>[4x]MKLVATLSSPEELELAEKADVVELRIDLFDFSGARVDKEKILTCRR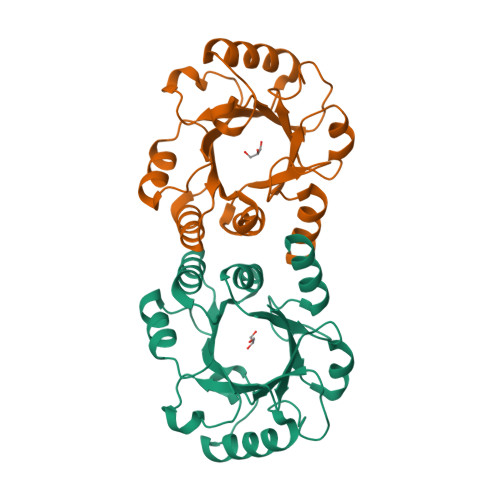VSDGGKFEGDERERIEKMKRAFDSLNPDYVDLESDLPDSAFDFNCRIIESYHNFIRTPDYSELKGIVEGRRGDLVKIATMGKSKRDVETIVRILTNYDDVVAFLMGERFSFTRVLAAYLGSPFIYCYVGSPKAPGQISLDDAREIISRLG>[3x]ESQLDLRVQELIKLICNVQAMEEMMMEMKYNTKKAPLGKLTVA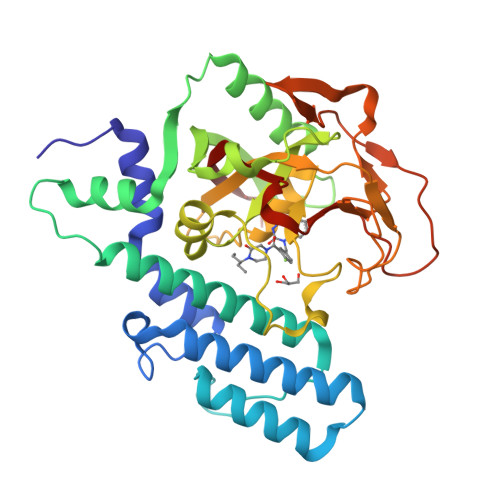QIKAGYQSLKKIEDCIRAGQHGRALMEACNEFYTRIPHDFGLRTPPLIRTQKELSEKIQLLEALGDIEIAIKLVKSERQGLEHPLDQHYRNLHCALRPLDHESYEFKVISQYLQSTHAPTHSDYTMTLLDLFEVEKDGEKEAFREDLHNRMLLWHGSRMSNWVGILSHGLRIAPPEAPITGYMFGKGIYFADMSSKSANYCFASRLKNTGLLLLSEVALGQCNELLEANPKAEGLLQGKHSTKGLGKMAPSSAHFVTLNGSTVPLGPASDTGILNPDGYTLNYNEYIVYNPNQVRMRYLLKVQFNFLQ>[20x]SLINTKIKPFKNQAFKNGEFIEVTEKDTEGRWSVFFFYPADFAFVCPTELGDVADHYEELQKLGVDVYSVST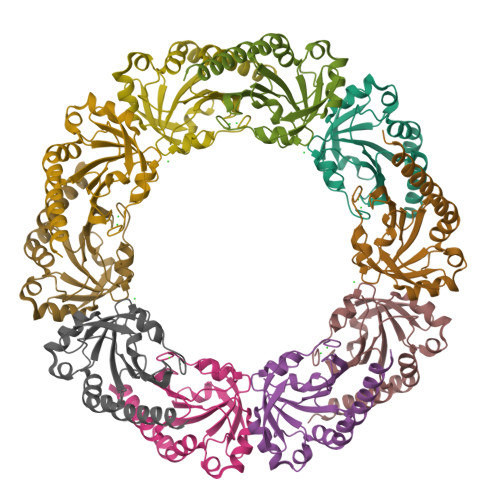DTHFTHKAWHSSSETIAKIKYAMIGDPTGALTRNFDNMREDEGLADRATFVVDPQGIIQAIEVTAEGIGRDASDLLRKIKAAQYVAAHPGEVCPAKWKEGEATLAPSLDLVGKI2-(4-NITROPHENYL)ACETIC ACID 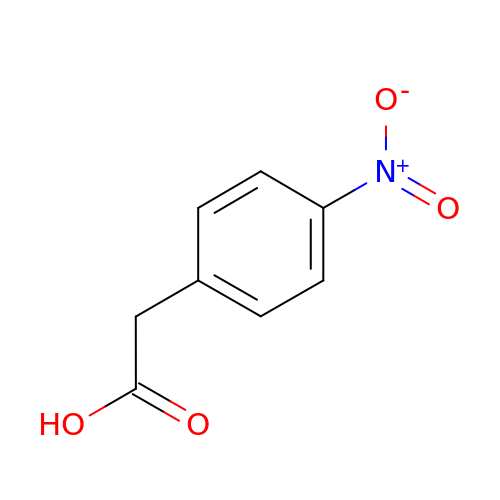| C8 H7 N O4 | YBADLXQNJCMBKR-UHFFFAOYSA-N> MLRQSLLSLAKVYGAVPPLGAAQGHRLLHGKREREGSLFAVANDVKRDERLLRQQLNALLEEERMPMQARLQRNEAVSSHEAVPQTPLVDLPGVERRRDLPADPITRLFFQHKGDHALYYGTYDKPSVQDDDRVQIEKRVPRRREENLYTPI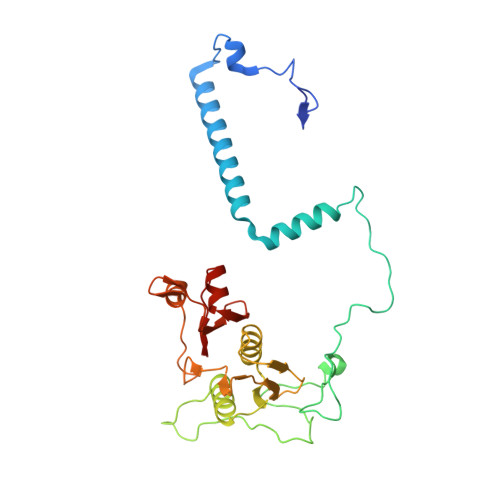YDFCHRIREATEQRKRFVVVPSTIETRGCARVMHDHGLVAGFRDFHNDRAFAVELKYFQGDSTINVIEPCSYDGRTEFEWSPKMMRRLLNTHGIHNRLVVYICRTADNRIIDHIHAVKENIGGRGLMMVH Basement membranes are extracellular structures of epithelia and endothelia that have collagen IV scaffolds of triple α-chain helical protomers that associate end-to-end, forming networks. At the C-termini, interactions occur between the trimeric NC1 domains of two protomers, forming a hexamer of these domains reinforced by sulfilimine cross-links. Recent studies in one of our laboratories revealed that the NC1 domains function as recognition modules, directing the selection and assembly of α-chains into protomers and networks.

Since all recombinant proteins used were prepared in NaCl buffers, and since hexamer assembly in the BM from bovine lens has recently been demonstrated to be chloride-dependent, the conformational changes observed in α2NC1homo and α4NC1homo that prevent chloride binding may hinder the final protomer–protomer assembly. Our findings of noncanonical assemblies for α2NC1 and α4NC1 homo-oligomers and the structural changes observed in the chains forming these noncanonical protomers in comparison to α2NC1α121 and to the chains in α1NC1homo, α3NC1homo and α5NC1homo could imply that chain folding is closely related to protomer assembly. It is unlikely that α2NC1homo and α4NC1homo could represent stable physio­logical assemblies, but the structures of the individual chains in these noncanonical oligomers might provide a frozen glimpse of transient conformational states in the process of NC1 folding and hexamer building.

>[6x]GYLGGFLLVLHSQTDQEPTCPLGMPRLWTGYSLLYLEGQEKAHNQDLGLAGSCLPVFSTLPFAYCNIHQVCHYAQRNDRSYWLASAAPLPMMPLSEEAIRPYVSRCAVCEAPAQAVAVHSQDQSIPPCPQTWRSLWIGYSFLMHTGAGDQGGGQALMSPGSCLEDFRAAPFLECQGRQGTCHFFANKYSFWLTTVKADLQFSSAPAPDTLKESQAQRQKISRCQVCVKYS> MTFRNCVAVDLGASSGRVMLARYERECRSLTLREIHRFNNGLHSQNGYVTWDVDSLESAIRLGLNKVCAAGIAIDSIGIDTWGVDFVLLDQQGQRVGLPVAYRDSRTNGLMAQAQQQLGKRDIYQRSGIQFLPFNTLYQLRALTEQQPELIPHIAHALLMPDYFSYRLTGKMNWEYTNATTTQLVNINSDDWDESLLAWSGANKAWFGRPTHPGNVIGHWICPQGNEIPVVAVASHDTASAVIASPLNGSRAAYLSSGTWSLMGFESQTPFTNDTALAANITNEGGAEGRYRVLKNIMGLWLLQRVLQERQINDLPALIAATQALPACRFIINPNDDRFINPDE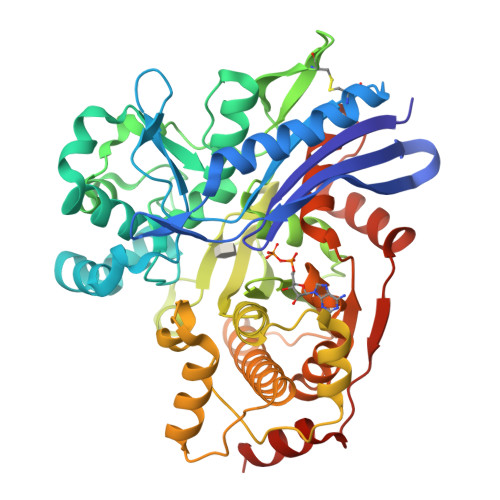MCSEIQAACREMAQPIPESDAELARCIFDSLALLYADVLHELAQLRGEDFSQLHIVGGGCQNTLLNQLCADACGIRVIAGPVEASTLGNIGIQLMTLDELNNVDDFRQVVSTTANLTTFTPNPDSEIAHYVALIHSTRQTKELCA> MDLKILSLATDKTTDKLQEFLQTLKDDDLASLLQNQAVKGRAVGTLLRAVLKGSPCSEEDGALRRYKIYSCCIQLVESGDLQQDVASEIIGLLMLEVHHFPGPLLVDLASDFVGAVREDRLVNGKSLELLPIILTALATKKEVLACGKGDLNGEEYKRQLIDTLCSVRWPQRYMIQLTSVFKDVCLTPEEMNLVVAKVLTMFSKLNLQEIPPLVYQLLVLSSKGSRRSVLDGIIAFFRELDKQHREEQSSDELSELITAPADELYHVEGTVILHIVFAIKLDCELGRELLKHLKAGQQGDPSKCLCPFSIALLLSLTRIQRFEEQVFDLLKTSVVKSFKDLQLLQGSKFLQTLVPQRTCVSTMILEVVRNSVHSWDHVTQGLIEFGFILMDSYGPKKILDGKAVEIGTSLSKMTNQHACKLGANILLETFKIHEMIRQEILEQVLNRVVTRTSSPINHFLDLFSDIIMYAPLILQNCSKVTETFDYLTFLPLQTVQGLLKAVQPLLKISMSMRDSLILVLRKAMFASQLDARKSAVAGFLLLLKNFKVLGSLPSSQCTQSIGVTQ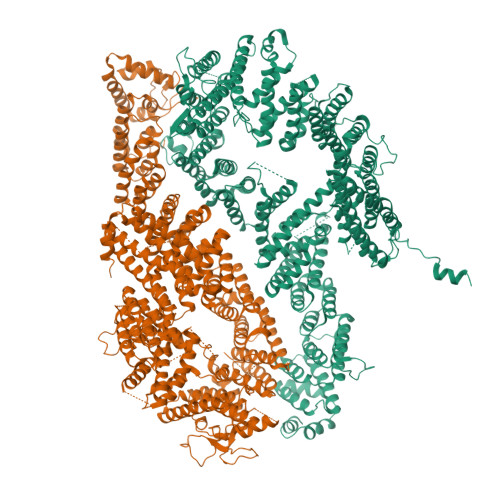VRVDVHSRYSAVANETFCLEIIDSLKRSLGQQADIRLMLYDGFYDVLRRNSQLASSIMQTLFSQLKQFYEPEPDLLPPLKLGACVLTQGSQIFLQEPLDHLLSCIQHCLAWYKSRVVPLQQGDEGEEEEEELYSELDDMLESITVRMIKSELEDFELDKSADFSQNTNVGIKNNICACLIMGVCEVLMEYNFSISNFSKSKFEEILSLFTCYKKFSDILSEKAGKGKAKMTSKVSDSLLSLKFVSDLLTALFRDSIQSHEESLSVLRSSGEFMHYAVNVTLQKIQQLIRTGHVSGPDGQNPDKIFQNLCDITRVLLWRYTSIPTSVEESGKKEKGKSISLLCLEGLQKTFSVVLQFYQPKVQQFLQALDVMGTEEEEAGVTVTQRASFQIRQFQRSLLNLLSSEEDDFNSKEALLLIAVLSTLSRLLEPTSPQFVQMLSWTSKICKEYSQEDASFCKSLMNLFFSLHVLYKSPVTLLRDLSQDIHGQLGDIDQDVEIEKTDHFAVVNLRTAAPTVCLLVLSQAEKVLEEVDWLIAKIKGSANQETLSDKVTPEDASSQAVPPTLLIEKAIVMQLGTLVTFFHELVQTALPSGSCVDTLLKGLSKIYSTLTAFVKYYLQVCQSSRGIPNTVEKLVKLSGSHLTPVCYSFISYVQNKSSDAPKCSEKEKAAVSTTMAKVLRETKPIPNLVFAIEQYEKFLIQLSKKSKVNLMQHMKLSTSRDFKIKGSVLDMVLREDEEHHHHHH;> SHNSHEVEENGSVFVKLLKASGLTLKTGENQNQLGVDQVIFQRKLFQALRKHPAYPKVIEEFVNGLESYTEDSESLRNCLLSCERLQDEEASMGTFYSKSLIKLLLGIDILQPAIIKMLFEKVPQFLFESENRDGINMARLIINQLKWLDRIVDGKDLTAQMMQLISVAPVNLQHDFITSLPEILGDSQHANVGKELGELLVQNTSLTVPILDVFSSLRLDPNFLSKIRQLVMGKLSSVRLEDFPVIVKFLLHSVTDTTSLEVIAELRENLNVQQFILPSRIQASQSKLKSKGLASSSGNQENSDKDCIVLVFDVIKSAIRYEKTISEAWFKAIERIESAAEHKSLDVVMLLIIYSTSTQTKKGVEKLLRNKIQSDCIQEQLLDSAFSTHYLVLKDICPSILLLAQTLFHSQDQRIILFGSLLYKYAFKFFDTYCQQEVVGALVTHVCSGTEAEVDTALDVLLELIVLNASAMRLNAAFVKGILDYLENMSPQQIRKIFCILSTLAFSQQPGTSNHIQDDMHLVIRKQLSSTVFKYKLIGIIGAVTMAGIMAEDRSVPSNSSQRSANVSSEQRTQVTSLLQLVHSCTEHSPWASSLYYDEFANLIQERKLAPKTLEWVGQTIFNDFQDAFVVDFCAAPEGDFPFPVKALYGLEEYSTQDGIVINLLPLFYQECAKDASRATSQESSQRSMSSLCLASHFRLLRLCVARQHDGNLDEIDGLLDCPLFLPDLEPGEKLESMSAKDRSLMCSLTFLTFNWFREVVNAFCQQTSPEMKGKVLSRLKDLVELQGILEKYLAVIPDYVPPFASVDLDTLDMMPRKTFVSLQNYRAFFRELDIEVFSILHSGLVTKFILDTEMHTEATEVVQLGPAELLFLLEDLSQKLENMLTAPFAKRICCFKNKGRQNIGFSHLHQRSVQDIVHCVVQLLTPMCNHLENIHNFFQCLGAEHLSADDKARATAQEQHTMACCYQKLLQVLHALFAWKGFTHQSKHRLLHSALEVLSNRLKQMEQDQPLEELVSQSFSYLQNFHHSVPSFQCGLYLLRLLMALLEKSAVPNQKKEKLASLAKQLLCRAWPHGEKEKNPTFNDHLHDVLYIYLEHTDNVLKAIEEITGVGVPELVSAPKDAASSTFPTLTRHTFVIFFRVMMAELEKTVKGLQAGTAADSQQVHEEKLLYWNMAVRDFSILLNLMKVFDSYPVLHVCLKYGRRFVEAFLKQCMPLLDFSFRKHREDVLSLLQTLQLNTRLLHHLCGHSKIRQDTRLTKHVPLLKKSLELLVCRVKAMLVLNNCREAFWLGTLKNRDLQGEEIISQDPSSSESNAEDSEDG> LTEGNPRWEQTH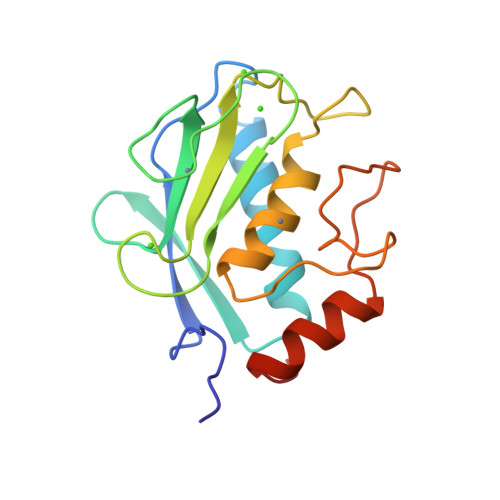LRYRIENYTPDLPRADVDHAIEKAFQLWSNVTPLTFTKVSEGQADIMISFVRGDHRDNSPFDGPGGNLAHAFQPGPGIGGDAHFDEDERWTNNFREYNLHRVAAHELGHSLGLSHSTDIGALMYPSYTFSGDVQLAQDDIDGIQAIYGRSQNPVQP> RKLILFIVFLALLLDNMLLTVVVPIIPSYLYSIKHEKNATEIQTARPVHTASISDSFQSIFSYYDNSTMVTGNATRDLTLHQTATQHMVTNASAVPSDCPSEDKDLLNENVQVGLLFASKATVQLITNPFIGLLTNRIGYPIPIFAGFCIMFVSTIMFAFSSSYAFLLIARSLQGIGSSCS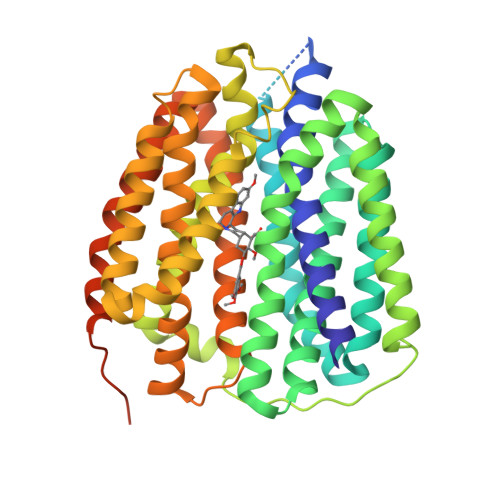SVAGMGMLASVYTDDEERGNVMGIALGGLAMGVLVGPPFGSVLYEFVGKTAPFLVLAALVLLDGAIQLFVLQPSRVQPESQKGTPLTTLLKDPYILIAAGSICFANMGIAMLEPALPIWMMETMCSRKWQLGVAFLPASISYLIGTNIFGILAHKMGRWLCALLGMIIVGVSILCIPFAKNIYGLIAPNFGVGFAIGMVDSSMMPIMGYLVDLRHVSVSGSVYAIADVAFCMGYAIGPSAGGAIAKAIGFPWLMTIIGIIDILFAPLCFFLRSPPAKEEKMAILMDHNCPIKTKMYTQNNIQSYPIGEDEESESD> MKNNHLLKSILLWGAVCIIVLAGPLSAFAASSSNPSDKLYFKNKKYYIFNNVWGADQVSGWWQTIYHNSDSDMGWVWNWPSNTSTVKAYPSIVSGWHWTEGYTAGSGFPTRLSDQKN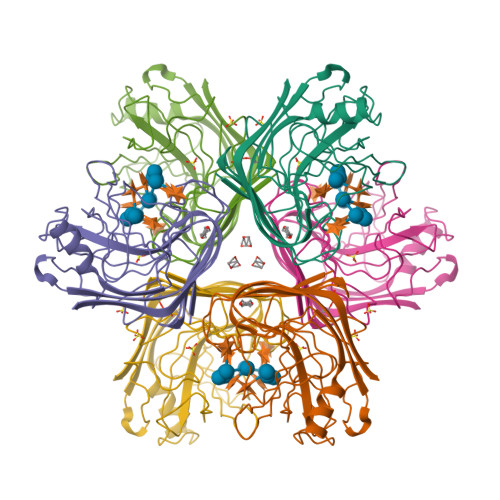INTKVSYSISANGTYNAAYDIWLHNTNKASWDSAPTDAIMIWLNNTNAGPAGSYVETVSIGGHSWKVYKGYIDAGGGKGWNVFSFIRTANTQSANLNIRDFTNYLADSKQWLSKTKYVSSVEFGTEVFGGTGQINISNWDVTVR> SLMSVPAIAPRRKRLADGLSVTQKVFVRSRNGGATKIVREHYLRSDIPCLSRSCTKCPQIVVPDAQNELPKFILSDSPLELSAPIGKHYVVLDTNVVLQAIDLLENPNCFFDVIVPQIVLDEVRNKSYPVYTRLRTLCRDSDDHKRFIVFHNEFSEHTFVERLPNETINDRNNRAIRKTCQWYSEHLKPYDINVVLVTNDRLNREAATKEVESNIITKSLVQYIELLPNADDIRDSIPQMDSFDKDLERDTFSDFTFPEYYSTARVMGGLKNGVLYQGNIQISEYNFLEGSVSLPRFSKPVLIVGQKNLNRAFNGDQVIVELLPQSEWKAPSSIVLDSEHFDVNDNPDIEAGDDDDNNESSSNTTVISDKQRRLLAKDAMIAQRSKKIQPTAKVVYIQRRSWRQYVGQLAPSSVDPQSSSTQNVFVILMDKCLPKVRIRTRRAAELLDKRIVISIDSWPTTHKYPLGHFVRDLGTIESAQAETEALLLEHDVEYRPFSKKVLECLPAEGHDWKAPTKLDDPEAVSKDPLLTKRKDLRDKLICSIDPPGCVDINDALHAKKLPNGNWEVGVHIADVTHFVKPGTALDAEGAARGTSVYLVDKRIDMLPMLLGTDLCSLKPYVDRFAFSVIWELDDSANIVNVNFMKSVIRSREAFSYEQAQLRIDDKTQNDELTMGMRALLKLSVKLKQKRLEAGALNLASPEVKVHMDSETSDPNEVEIKKLLATNSLVEEFMLLANISVARKIYDAFPQTAMLRRHAAPPSTNFEILNEMLNTRKNMSISLESSKALADSLDRCVDPEDPYFNTLVRIMSTRCMMAAQYFYSGAYSYPDFRHYGLAVDIYTHFTSPIRRYCDVVAHRQLAGAIGYEPLSLTHRDKNKMDMICRNINRKHRNAQFAGRASIEYYVGQVMRNNESTETGYVIKVFNNGIVVLVPKFGVEGLIRLDNLTEDPNS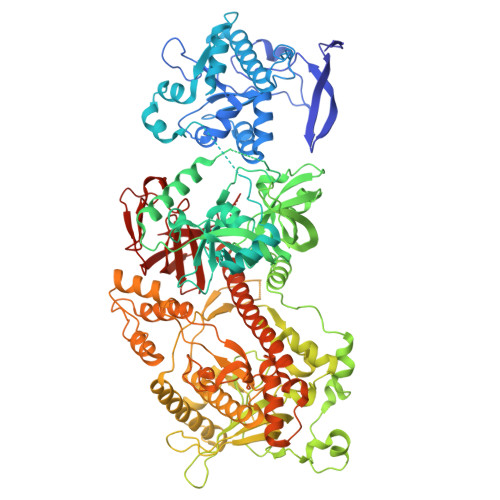AAFDEVEYKLTFVPTNSDKPRDVYVFDKVEVQVRSVMDPITSKRKAELLLK>[3x]SMTGAVCPGSFDP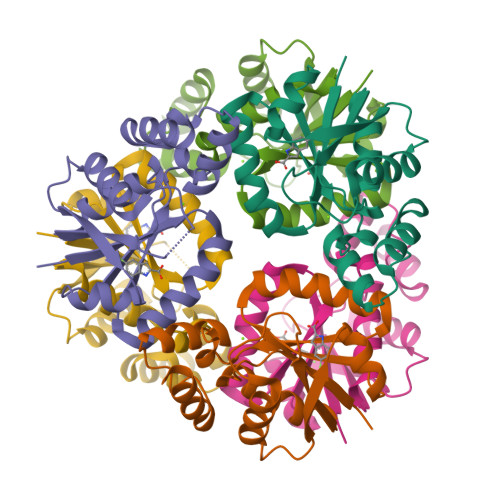VTLGHLDVFERAAAQFDEVIVAVLINPNKAGMFTVDERIEMIRESTADLPNLRVESGQGLLVDFVRERGLNAIVKGLRTGTDFEYELQMAQMNKHIAGVDTFFVATAPAYSFVSSSLAKEVATYGGDVSALLPASVHQRLLGKLRGQAQ5-(1-ethoxyisoquinolin-3-yl)-2,4-dihydro-3H-1,2,4-triazol-3-one 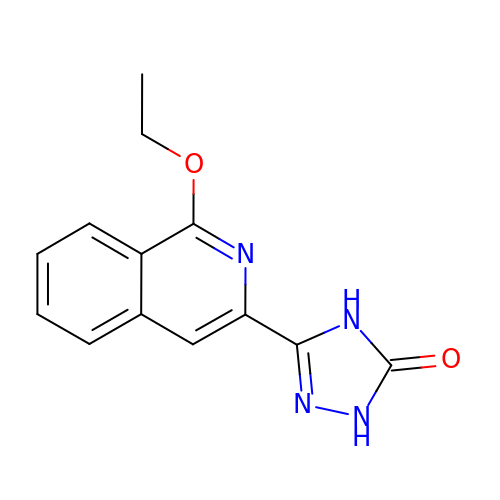| C13 H12 N4 O2 | RHTTUBBYQVKYBV-UHFFFAOYSA-N>GSHMGQELVSLEGHQSAITALAFSKNIVVSG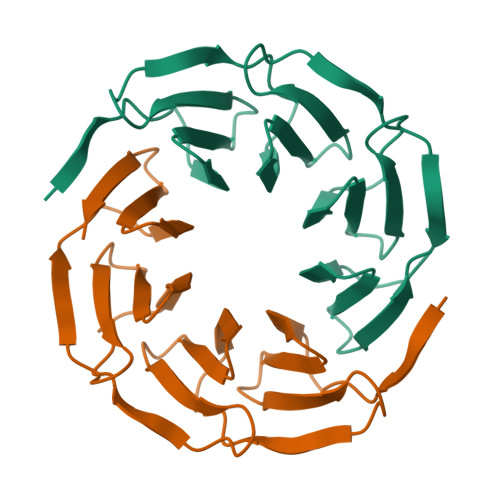AADGTIKVWDILTGQLLRDHDGHQSEVTALQFKDNIVVSGAKDGTVKVWYIGTGQELVSLEGHQSAITALAFSKNIVVSGAADGTIKVWDILTGQLLRDHDGHQSEVTALQFKDNIVVSGAKDGTVKVWYIGT[12x]> VGTQTGNPATNLPEAQGSASKEAEQSQNQAGETNGSIPVEVPKTDLDQAAKD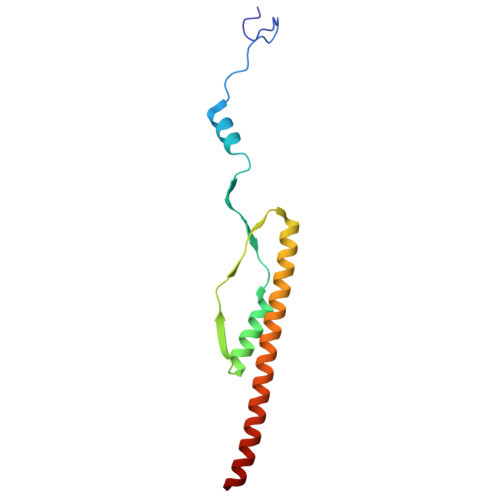AKSAGVNVVQDADVNKGTVKTAEEAVQKETEIKEDYTKQAEDIKKTTDQYKSDVAAHEAEVAKIKAKNQ>GAHMSYSYDAPSDFINFSSKQKNEESKKRQWALEDFEIGRPLGKGKFGNVYLAREKQSKFILALKVLFKAQLEKAGVEHQLRREVEIQSHLRHPNILRLYGYFHDATRVYLILEYAPLGTVYRELQKLSKFDEQRTATYITELANALSYCHSKRVIHRDIKPE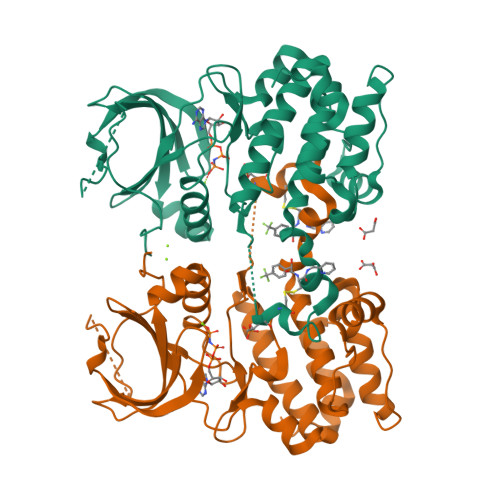NLLLGSAGELKIADFGWSVHAPSSRRTTLCGTLDYLPPEMIEGRMHDEKVDLWSLGVLCYEFLVGKPPFEANTYQETYKRISRVEFTFPDFVTEGARDLISRLLKHNPSQRPMLREVLEHPWITANSSK[2x]3-[(2-amino-4-methylquinolin-7-yl)methoxy]-5-[2-(methylamino)ethyl]benzonitrile | 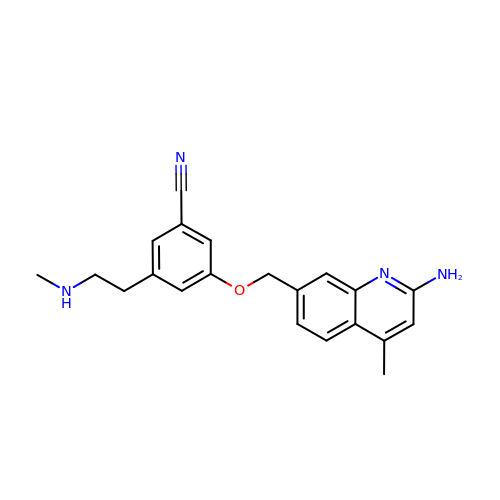C21 H22 N4 O | QKCPYJJSYKWGHS-UHFFFAOYSA-N>[2x]GPLGSNRRLQQTQAQVDEVVDIMRVNVDKVLERDQKL;>[2x]GSALSEIETRHSEIIKL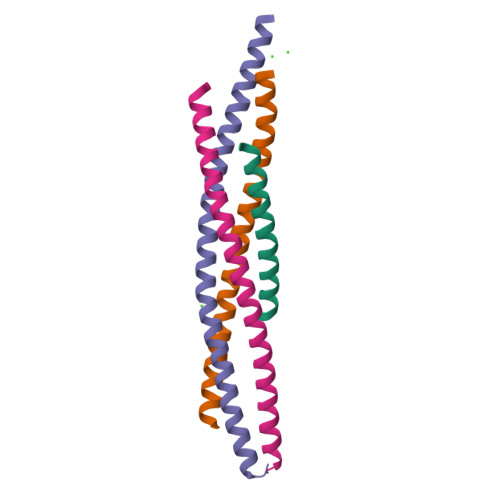ENSIRELHDMFMDMAMLVESQGEMIDRIEYNVEHAVDYVERAVSDTKK;>[2x]GSHMMRNELEEMQRRADQLADESLESTRRMLQLVEESKDAGIRTLVMLDEQGEQLDRVEEGMNHINQDMKEAEKNLKDLGW;>GSARENEMDENLEQVSGIIGNLRHMALDMGNEIDTQNRQIDRIMEKADSNKTRIDEANQRATKML[2x]>MTTAVENIQVAEITPSTRIVYRGVSPAEFIYLEGNKFSRAQSPTQGNDDPQWKALYTGSDANVSSRNITDNPGGVVKIEYPSDWKVLEITSTTPSQKWHNDMGEAWPVWRAVKKWAASNQVDLPDVTASNIDDYLLLDELGKKKIILKKPIGEDDVSSHEFIIPWKMAETVAQNKIDSTSDPAAKFFTPDDLDSTTKQPKDQAAVRRILKKWDAYSCKGGASATFGVASLCGINVAAYKADIEKLIKDVYEDPNFSDLKNRTGGPQKDKDTLKGYYERLKPKVETLRPLKAGVSSAVGAAGAIS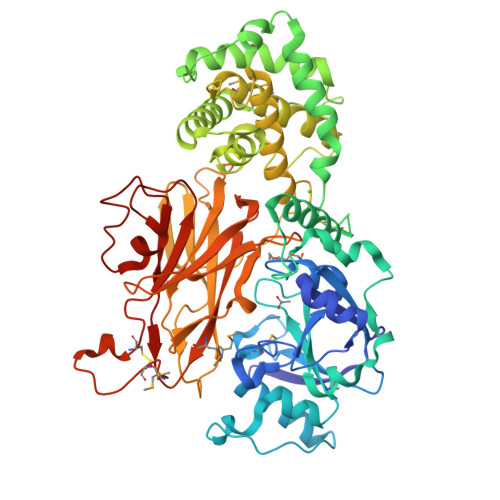WAIGVADAFTSENVSSFDKAAAVTAIVPGLGECVGIANAIDKRDPEGLIINTISMAALMASAAVPVLAPIGVALDAGLAAAQGVATVLEYLEIGQPARTPLPVSSPKTHKGVTAAWVGSERIIAHRPRPGMRQHIFSVSIDSSKPEYTAPLIEVAGVRADGKLDPSPEWIRIRQNHYPIPFRFEKLSGDSPYAFRCVLLRPTTITRTEPVYVTFAYMTSDMTCRTGESDPNKACSPNNPAIAVRFGSLVKNEDERSVLAVTWPGPSIRPETNWIKLPYSIHPY[4x]> GAMAEEQMRLPSADVYRFAEPDSEENIIFEENMQPKAGIPIIKAGTVIKLIERLTYHMYADPNFVRTFLTTYRSFCKPQELLSLIIERFEIPEPEPTEADRIAIENGDQPLSAELKRFRKEYIQPVQLRVLNVCRHWVEHHFYDFERDAYLLQRMEEFIGTVRGKAMKKWVESITKIIQRKKIARDNGPGHNITFQSSPPTVEWHISRPGHIETFDLLTLHPIEIARQLTLLESDLYRAVQPSELVGSVWTKEDKEINSPNLLKMIRHTTNLTLWFEKCIVETENLEERVAVVSRIIEILQVFQE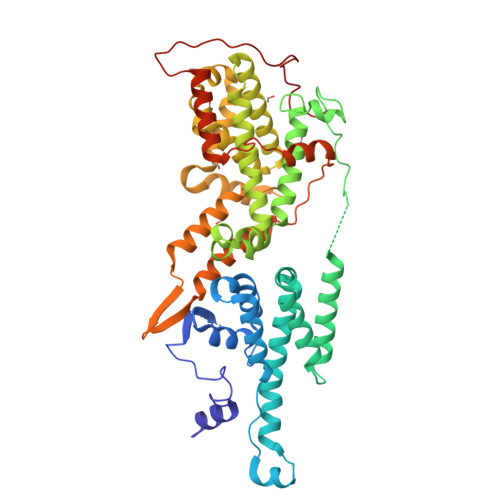LNNFNGVLEVVSAMNSSPVYRLDHTFEQIPSRQKKILEEAHELSEDHYKKYLAKLRSINPPCVPFFGIYLTNILKTEEGNPEVLKRHGKELINFSKRRKVAEITGEIQQYQNQPYCLRVESDIKRFFENLNPMGNSMEKEFTDYLFNKSLEIEPRNPKPLPRFPKKYSYPLKSPGVRPSNPRPGT>GHPETLVKVKDAEDQLGARVGYIELDLNSGKILESFRPEERFPMMSTFKVLLCGAVLSRVDAGQEQLGRRIHYSQNDLVEYSPVTEKHLTDGMTVRELCSAAITMSDNTAANLLLTTIGGPKELTAFLHNMGDHVTRLDRWEPELNEAIPNDERDTTTPAAMATTLRKLLTGELLTLASRQQLIDWMEADKVAGP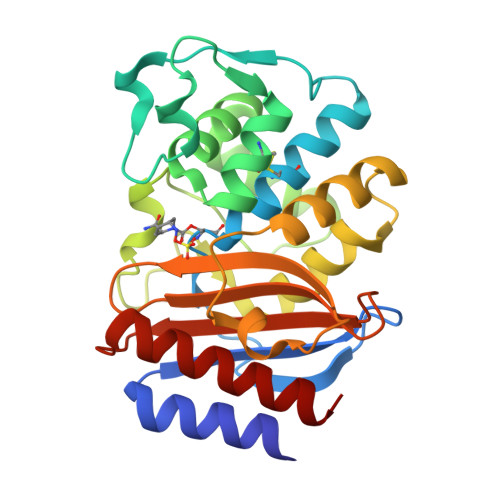LLRSALPAGWFIADKSGAGERGSRGIIAALGPDGKPSRIVVIYTTGSQATMDERNRQIAEIGASLIKHW[4x]> MDVVDPDIFNRDPRDHYDLLQRLGGGTYGEVFKARDKVSGDLVALKMVKMEPDDDVSTLQKEILILKTCRHANIVAYHGSYLWLQKLWICMEFCGAGSLQDIYQVTGSLSELQISYVCREVLQGLAYLHSQKKIHRDIKGANILINDAGEVRLADFGISAQIGAELARRLEFIGTPYWMAPEVAAVALKGGYNELCDIWSLGITAIE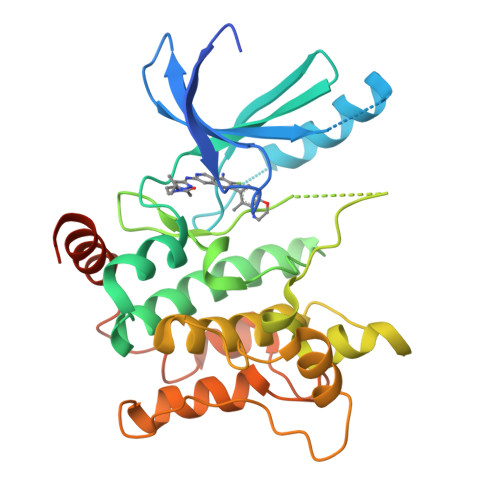LAELQPPLFDVHPLRVLFLMTKSGYQPPRLKEKGKWSAAFHNFIKVTLTKSPKKRPSATKMLSHQLVSQPGLNRGLILDLLDKLKNPGKGPSIGDIEDEE> MGATDRTPPSNAILSNSNSDNNSTQGSQSGTVTKTPNPEATGSLSGKPTQIPPLSDEVTTRSLIRENQSAVTLANKGYDVVQNPEVLGPKNPDYTINGQVFDNYAPATGNVRNIATTISNK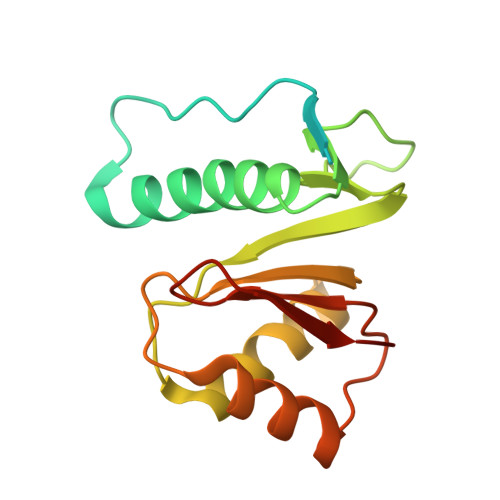VSSGQASNIVVNLADSSASPAAIEAQINSYPIPGLGKVIVIDKLGNITIIKPKGN>MQRLFLLVAVMLLSGCLTAPPKEAARPTLMPRAQSYKDLTHLPAPTGKIFVSVYNIQDETGQFKPYPASNFSTAVPQSATAMLVTALKDSRWFIPLERQGLQNLLNERKIIRAAQENGTVAINNRIPLQSLTAANIMVEGSIIGYESNVKSGGVGARYFGIGADTQYQLDQIAVNLRVVNVSTGEILSSVNTSKTILSYEVQAGVFRFIDYQRLLEGEVGYTSNEPVMLCLMSAIETGVIFLINDGIDRGLWDLQNKAERQNDILVKYRHMSVPPES[9x];>[9x]MRVKHAVVLLMLISPLSWAGTMTFQFRNPNFGGNPNNGAFLLNSAQAQNSYKDPSYNDDFGIETPSALDNFTQAIQSQILGGLLSNINTGKPG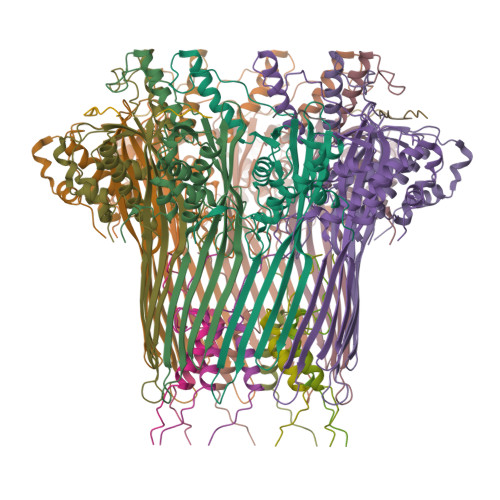RMVTNDYIVDIANRDGQLQLNVTDRKTGQTSTIQVSGLQNNSTDF;>GVVPQYGGGGNHGGGGNNSGPN[9x]>[2x]GSVVIVGRIILSGSGSITAYSQQTRGLLGCIITSLTGRDKNQVEGEVQVVSTATQSFLATCVNGVCWTVYHGAGSKTLAGPKGPITQMYTNVDQDLVGWQAPPGARSLTPCTCGSSDLYLVTRHADVIPVRRRGDSRGSLLSPRPVSYLKGSSGGPLLCPSGHAVGIFRAAVCTRGVAKAVDFVPVESMETTMRSPVFTDNSSPPAVPQSFQVAHLHAPTGSGKSTKVPAAYAAQGYKVLVLNPSVAATLGFGAYMSKAHGIDPNIRTGVRTITTGAPVTYSTYGKFLADGGCSGGAYDIIICDECHSTDSTTILGIGTVLDQAETAGARLVVLATATPPGSVTVPHPNIEEVALSNTGEIPFYGKAIPIEAIRGGRHLIFCHSKKKCDELAAKLSGLGINAVAYYRGLDVSVIPTIGDVVVVATDALMTGYTGDFDSVIDCN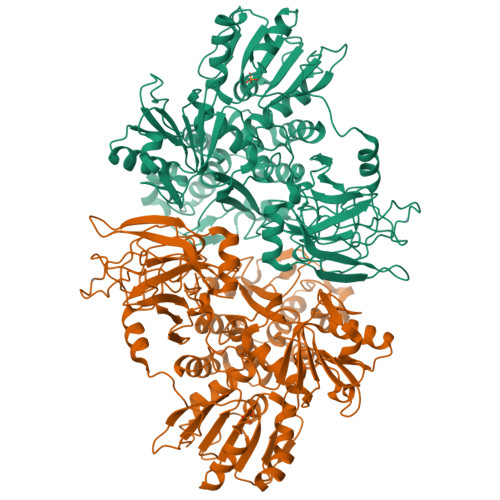TCVTQTVDFSLDPTFTIETTTVPQDAVSRSQRRGRTGRGRRGIYRFVTPGERPSGMFDSSVLCECYDAGCAWYELTPAETSVRLRAYLNTPGLPVCQDHLEFWESVFTGLTHIDAHFLSQTKQAGDNFPYLVAYQATVCARAQAPPPSWDQMWKCLIRLKPTLHGPTPLLYRLGAVQNEVTLTHPITKYIMACMSADLEVVT> ADDIVLKAKNGDVKFPHKAHQKAVPDCKKCHEKGPGKIEGFGKEMAHGKGCKGCHEEDKKG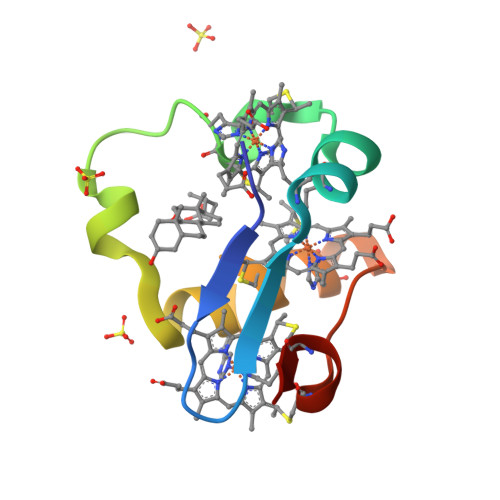PTKCGECHKK> XIAEQLRRI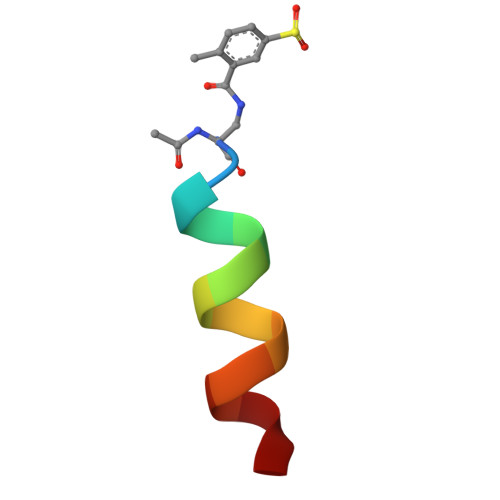GDRF>DYKDDDDKLVPRGSCHPRLSLHRPALEDLLLGSEANLTCTLTGLRDASGVTFTWTPSSGKSAVQGPPERDLCGCYSVSSVLPGCAEPWNHGKTFTCTAAYPESKTPLTATLSKSGNTFRPEVHLLPPPSEELALNELVTLTCLARGFSPKDVLVRWLQGSQELPREKYLTWASRQEPSQGTTTFAVTSILRVAAEDWKKGDTFSCMVGHEALPLAFTQKTIDRLAGKPTHVNVSVVMAEVDGTCY[4x];> KSPIFGPEEVNSVEGNSVSITCYYPPTSVNRHTRKYWCRQGARGGCITLISSEGYVSSKYAGRANLTNFPENGTFVVNIAQLSQDDSGRYKCGLGINSRGLSFDVSLEVSQGPGLLNDTKVYTVDLGRTVTINCPFKTENAQKRKSLYKQIGLYPVLVIDSSGYVNPNYTGRIRLDIQGTGQLLFSVVINQLRLSDAGQYLCQAGDDSNSNKKNADLQVLKPEPELVYEDLRGSVTFHCALGPEVANVAKFLCRQSSGENCDVVVNTLGKRAPAFEGRILLNPQDKDGSFSVVITGLRKEDAGRYLCGAHSDGQLQEGSPIQAWQLFVNEESTIPRSPTVVKGVAGGSVAVLCPYNRKESKSIKYWCLWEGAQNGRCPLLVDSEGWVKAQYEGRLSLLEEPGNGTFTVILNQLTSRDAGFYWCLTNGDTLWRTTVEIKIIEGEPNLKVPGNVTAVLGETLKVPCHFPCKFSSYEKYWCKWNNTGCQALPSQDEGPSKAFVNCDENSRLVSLTLNLVTRADEGWYWCGVKQGHFYGETAAVYVAVEERKAAGSRDVSLAKAD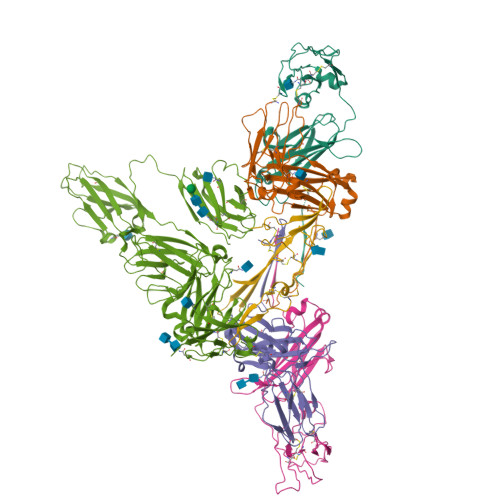AAPDEKVLDSGFREIENKAIQDPRHHHHHH;> QEDERIVLVDNKCKCARITSRIIRSSEDPNEDIVERNIRIIVPLNNRENISDPTSPLRTRFVYHLSDLCKKCDPTEVELDNQIVTATQSNICDEDSATETCYTYDRNKCYTAVVPLVYGGETKMVETALTPDACYPD> GDVTFDVGDEYEIIETIGNGAYGVVSSARRRLTGQQVAIKKIPNAFDVVTNAKRTLRELKILKHFKHDNIIAIKDILRPTVPYGEFKSVYVVLDLMESDLHQIIHSSQPLTLEHVRYFLYQLLRGLKYMHSAQVIHRDLKPSNLLVNENCELKIGDFGMARGLCTSPAEHQYFMTEYVATRWYRAPELMLSLHEYTQAIDLWSVGCIFGEMLARRQLFPGKNYVHQLQLIMMVLGTPSPAVIQAVGAERVRAYIQSLPPRQPVPWETVYPGADRQALSLLGRMLRFEPSARISAAAALRHPFLAKYHDPDDEPDCAPP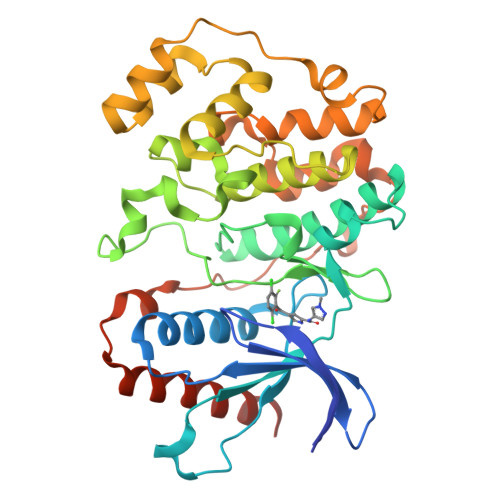FDFAFDREALTRERIKEAIVAEIEDFHARREGIRQQIRFQ>GSFTGVIIKQGCLLKQGHRRKNWKVRKFILREDPAYLHYYDPAGAEDPLGAIHLRGCVVTSVESNSNGRKSEEEN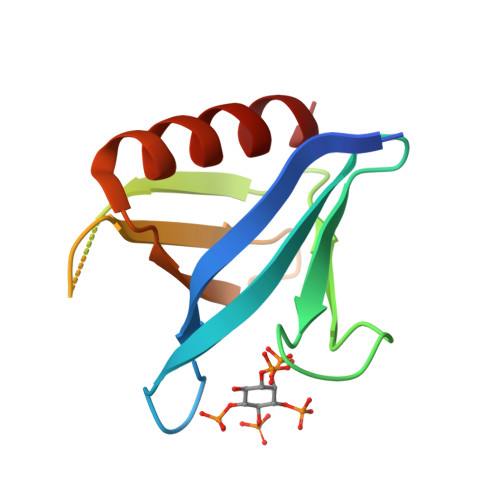LFEIITADEVHYFLQAATPKERTEWIKAIQMASR[3x]(1S)-N-{[3-(diphenylmethyl)-1,2,4-oxadiazol-5-yl]methyl}-N-methyl-1-(thiophen-2-yl)ethan-1-amine | C23 H23 N3 O S | 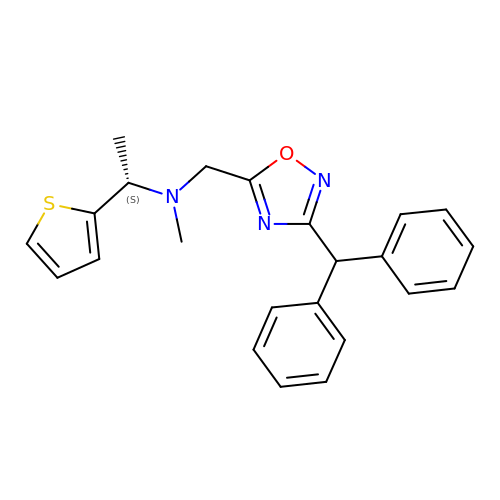YMVZNLFSCPAPNW-KRWDZBQOSA-N> GLGQMLESMIDNTVRETVGAATSRDALPNTEASGPTHSKEIPALTAVETGATNPLVPSDTVQTRHVVQHRSRSESSIESFFARGACVTIMTVDNPASTTNKDKLFAVWKITYKDTVQLRRKLEFFTYSRFDMELTFVVTANFTETNNGHALNQVYQIMYVPPGAPVPEKWDDYTWQTSSNPSIFYTYGTAPARISVPYVGISNAYSHFYDGFSKVPLKDQSAALGDSLYGAASLNDFGILAVRVVNDPNPTKVTSKIRVYLKPKHIRVWCPRPPRAVAYYGPGVDYKDGTLTPLSTKDLTTY;> MGAQVSSQKVGAHENSNGAYGGSTINYTTINYYRDSASNAASKQDFSQDPSKFTEPIKDVLIKTAPMLNSPNIEACGYSDRVLQLTLGNSTITAQEAANSVVAYGRWPEYLRDSEANPVDQPTEPEVAACRFYTLDTVSWTKESRGWWWKLPDALRDMGLFGQNMYYHYLGRSGYTVHVQCNASKFHQGALGVFAVPEMCLAGDSNTTTMHTSYQNANPGEKGGTFTGTFTPDNNQTSPARRFCPVDYLLGNGTLLGNAFVFPHQIINLRTNNCATLV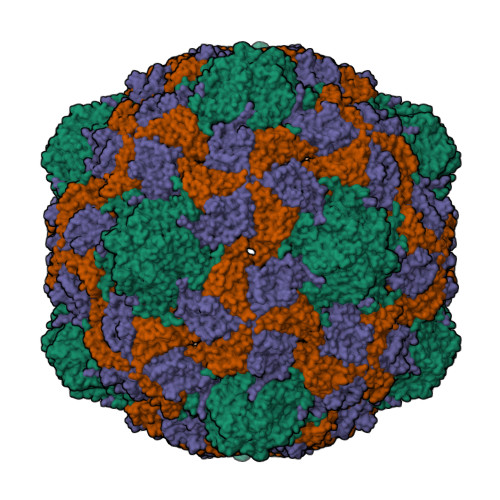LPYVNSLSIDSMVKHNNWGIAILPLAPLNFASESSPEIPITLTIAPMCCEFNGLRNITLPRLQ;> GLPVMNTPGSNQYLTADNFQSPCALPEFDVTPPIDIPGEVKNMMELAEIDTMIPFDLSATKKNTMEMYRVRLSDKPHTDDPILCLSLSPASDPRLSHTMLGEILNYYTHWAGSLKFTFMFCGSMMATGKLLVSYAPPGADPPKKRKEAMLGTHVIWDIGLQSSCTMVVPWISNTTYRLTIDDSFTEGGYISVFYQTRIVVPLSTPREMDILGFVSACNDFSVRLLRDTTHIEQKALAQ>MTGMSREEVESLIQEVLEVYPEKARKDRNKHLAVNDPAVTQSKKCIISNKKSQPGLMTIRGCAYAGSKGVVWGPIKDMIHISHGPVGCGQYSRAGRRNYYIGTTGVNAFVTMNFTSDFQEKDIVFGGDKKLAKLIDEVETLFPLNKGISVQSECPIGLIGDDIESVSKVKGAELSKTIVPVRCEGFRGVSQSLGHHIANDAVRDWVLGKRDEDTTFASTPYDVAIIGDYNIGGDAWSSRILLEEMGLRCVAQWSGDGSISEIELTPKVKLNLVHCYRSMNYISRHMEEKYGIPWMEYNFFGPTKTIESLRAIAAKFDESIQKKCEEVIAKYKPEWEAVVAKYRPRLEGKRVMLYIGGLRPRHVIGAYEDLGMEVVGTGYEFAHNDDYDRTMKEMGDSTLLYDDVTGYEFEEFVKRIKPDLIGSGIKEKFIFQKMGIPFREMHSWDYSGPYHGFDGFAIFARDMDMTLNNPCWKKLQAPWEASEGAEKVAASA[2x];>MSQQVDKIKASYPLFLDQDYKDMLAKKRDGFEEKYPQDKIDEVFQWTTTKEYQELNFQREALTVNPAKACQPLGAVLCALGFEKTMPYVHGSQGCVAYFRSYFNRHFREPVSCVSDSMTEDAAVFGGQQNMKDGLQNCKATYKPDMIAVSTTCMAEVIGDDLNAFINNSKKEGFIPDEFPVPFAHTPSFVGSHVTGWDNMFEGIARYFTLKSMDDKVVGSNKKINIVPGFETYLGNFRVIKRMLSEMGVGYSLLSDPEEVLDTPADGQFRMYAGGTTQEEMKDAPNALNTVLLQPWHLEKTKKFVEGTWKHEVPKLNIPMGLDWTDEFLMKVSEISGQPIPASLTKERGRLVDMMTDSHTWLHGKRFALWGDPDFVMGLVKFLLELGCEPVHILCHNGNKRWKKAVDAILAASPYGKNATVYIGKDLWHLRSLVFTDKPDFMIGNSYGKFIQRDTLHKGKEFEVPLIRIGFPIFDRHHLHRSTTLGYEGAMQILTTLVNSILERLDEETRGMQATDYNHDLVR[2x];> MSWRILLCHKHPVSARLRFLIPTGGGVVLPQTLPRLAVIAEDQEAPVQCHPASALRALQETMALGWQLELIGEFRLNMEVPGQIMPIYLAALAGHELPPPPEGTRWIELTQSIGMPWLDRELLRRVYEELIGFGC

Biological nitrogen fixation, performed by the enzyme nitrogenase, supplies nearly 50% of the bioavailable nitrogen pool on Earth, yet the structural nature of the enzyme intermediates involved in this cycle remains ambiguous. The MoFe-protein is a heterotetramer with the homologous α- and β-subunits forming an α2β2 dimer of αβ dimers. Sandwiched between the two subunits within an αβ dimer lies the intermediary [8Fe:7S] P-cluster. This cluster transfers electrons into the active site [7Fe:1Mo:9S:C]-R-homocitrate FeMo-cofactor positioned within the α-subunit.

The structure of the MoFe-protein purified from HCA-deficient cells (MoFe∆nifV) revealed an endogenous binding interaction with the protein nitrogenase associated factor T (NafT), of unknown function. Given the structural similarities between MoFe∆nifV and the alkaline inhibited states, we sought to determine if NafT can also recognize the MoFeAlkaline-inactivated state. Alkaline turnover reactions were performed for 4 h with and without NafT present, and subsequently subjected to concentration and S.E.C. before structural analysis. The cryoEM structure obtained from these samples revealed a 1:1 MoFeAlkaline-inactivated-NafT complex at 2.33 Å resolution with two disordered MoFe-protein αβ-dimers. Interestingly, both active sites contain identifiable density for the FeMo-cofactors in the resting state position, despite the apparent absence of density for the HCA. However, within the MoFe-protein of the MoFeAlkaline-inactivated-NafT structure, the residue α-Arg277 displays an altered conformation relative to the resting state and is positioned between the cofactor and NafT, blocking direct contact between NafT and the metallocluster. It is possible that NafT is indirectly stabilizing the FeMo-cofactor within the HCA-deficient active site through interactions at the interface between the α- and β- subunits, potentially precluding Fe-protein binding and thus preventing further turnover of a ‘damaged’ protein. We further demonstrate that the nitrogenase associated factor T protein can recognize and bind an alkaline inactivated MoFe-protein in vitro.>[4x]MLESKLKAPVFTATTQGDHYGEFVLEPLERGFGVTLGNPLRRILLSSIPGTAVTSVYIEDVLHEFSTIPGVKEDVVEIILNLKELVVRFLDPKMASTTLILRAEGPKEVRAGDFTPSADVEIMNPDLHIATLEEGGKLYMEVRVDRGVGYVPAERHGIKDRINAIPVDAIFSPVRRVAFQVEDTRLGQRTDLDKLTLRIWTDGSVTPLEALNQAVAILKEHLNYFANPEASLLPTPEVSKGEKRESAEEDLDLPLEELGLSTRVLHSLKEEGIESVRALLALNLKDLRNIPGIGERSLEEIRQALAKKGFTLKE;>[2x]MEIKRFGRIREVIPLPPLTEIQVESYKKALQADVPPEKRENVGIQAAFKETFPIEEGDKGKGGLVLDFLEYRIGDPPFSQDECREKDLTYQAPLYARLQLIHKDTGLIKEDEVFLGHLPLMTEDGSFIINGADRVIVSQIHRSPGVYFTPDPARPGRYIASIIPLPKRGPWIDLEVEASGVVTMKVNKRKFPLVLLLRVLGYDQETLVRELSAYGDLVQGLLDEAVLAMRPEEAMVRLFTLLRPGDPPKKDKALAYLFGLLADPKRYDLGEAGRYKAEEKLGVGLSGRTLVRFEDGEFKDEVFLPTLRYLFALTAGVPGHEVDDIDHLGNRRIRTVGELMADQFRVGLARLARGVRERMVMGSPDTLTPAKLVNSRPLEAALREFFSRSQLSQFKDETNPLSSLRHKRRISALGPGGLTRERAGFDVRDVHRTHYGRICPVETPEGANIGLITSLAAYARVDALGFIRTPYRRVKNGVVTEEVVYMTASEEDRYTIAQANTPLEGDRIATDRVVARRRGEPVIVAPEEVEFMDVSPKQVFSLNTNLIPFLEHDDANRALMGSNMQTQAVPLIRAQAPVVMTGLEERVVRDSLAALYAEEDGEVVKVDGTRIAVRYEDGRLVEHPLRRYARSNQGTAFDQRPRVRVGQRVKKGDLLADGPASEEGFLALGQNVLVAIMPFDGYNFEDAIVISEELLKRDFYTSIHIERYEIEARDTKLGPERITRDIPHLSEAALRDLDEEGIVRIGAEVKPGDILVGRTSFKGEQEPSPEERLLRSIFGEKARDVKDTSLRVPPGEGGIVVGRLRLRRGDPGVELKPGVREVVRVFVAQKRKLQVGDKLANRHGNKGVVAKILPVEDMPHLPDGTPVDVILNPLGVPSRMNLGQILETHLGLAGYFLGQRYISPVFDGATEPEIKELLAEAFNLYFGKRQGEGFGVDKREKEVLARAEKLGLVSPGKSPEEQLKELFDLGKVVLYDGRTGEPFEGPIVVGQMFIMKLYHMVEDKMHARSTGPYSLITQQPLGGKAQFGGQRFGEMEVWALEAYGAAHTLQEMLTIKSDDIEGRNAAYQAIIKGEDVPEPSVPESFRVLVKELQALALDVQTLDEKDNPVDIFEGLASKR;>MKKEVRKVRIALASPEKIRSWSYGEVEKPETINYRTLKPERDGLFDERIFGPIKDYECACGKYKRQRFEGKVCERCGVEVTRSIVRRYRMGHIELATPAAHIWFVKDVPSKIGTLLDLSATELEQVLYFNKYIVLDPKGAVLDGVPVEKRQLLTDEEYRELRYGKQETYPLPAGVDALVKDGEEVVKGQELAPGVVSRMDGVALYRFPRRVRVDYLRKERAALRIPLSAWVEKEAYRPGEVLAELSEPYLFRAEESGVVELKDLAEGHLIYLRQEEEVVARYFLPAGMTPLVVEGEIVEVGQPLAEGKGLLRLPRHMTAKEVEAEEEGDSVHLTLFLEWTEPKDYKVAPHMNVIVPEGAKVQAGEKIVAAIDPEEEVIAEAEGVVHLHEPASILVVKARVYPFEDDVEVTTGDRVAPGDVLADGGKVKSEIYGRVEVDLVRNVVRVVESYDIDARMGAEAIQELLKELDLEKLERELLEEMKHPSRARRAKARKRLEVVRAFLDSGNRPEWMILEAVPVLPPDLRPMVQVDGGRFATSDLNDLYRRLINRNNRLKKLLAQGAPEIIIRNEKRMLQEAVDAVIDNGRRGSPVTNPGSERPLRSLTDILSGKQGRFRQNLLGKRVDYSGRSVIVVGPQLKLHQCGLPKRMALELFKPFLLKKMEEKAFAPNVKAARRMLERQRDIKDEVWDALEEVIHGKVVLLNRAPTLHRLGIQAFQPVLVEGQSIQLHPLVCEAFNADFDGDQMAVHVPLSSFAQAEARIQMLSAHNLLSPASGEPLAKPSRDIILGLYYITQVRKEKKGAGMAFATPEEALAAYERGEVALNAPIVVAGRETSVGRLKFVFANPDEALLAVAHGLLDLQDVVTVRYLGRRLETSPGRILFARIVGEAVGDEKVAQELIQMDVPQEKNSLKDLVYQAFLRLGMEKTARLLDALKYYGFTLSTTSGITIGIDDAVIPEEKQRYLEEADRKLRQIEQAYEMGFLTDRERYDQVIQLWTETTEKVTQAVFKNFEENYPFNPLYVMAQSGARGNPQQIRQLCGMRGLMQKPSGETFEVPVRSSFREGLTVLEYFISSHGARKGGADTALRTADSGYLTRKLVDVAHEIVVREADCGTTNYISVPLFQMDEVTRTLRLRKRSDIESGLYGRVLAREVEALGRRLEEGRYLSLEDVHFLIKAAEAGEVREVPVRSPLTCQTRYGVCQKCYGYDLSMARPVSIGEAVGVVAAESIGEPGTQLTMRTFHTGGVAVGTDITQGLPRVIELFEARRPKAKAVISEIDGVVRIEEGEDRLSVFVESEGFSKEYKLPKDARLLVKDGDYVEAGQPLTRGAIDPHQLLEAKGPEAVERYLVDEIQKVYRAQGVKLHDKHIEIVVRQMLKYVEVTDPGDSRLLEGQVLEKWDVEALNERLIAEGKVPVAWKPLLMGVTKSALSTKSWLSAASFQNTTHVLTEAAIAGKKDELIGLKENVILGRLIPAGTGSDFVRFTQVVDQRTLKAIEEARKEAVEAKEKEAPRRPVRREQPGKGL[2x];>[2x]MAEPGIDKLFGMVDSKYRLTVVVAKRAQQLLRHRFKNTVLEPEERPKMRTLEGLYDDPNAVTWAMKELLTGRLFFGENLVPEDRLQKEMERLYPTEEEA;>[2x]TSDPVRQYLHEIGQVPLLTLEEEIDLARKVEEGMEAIKKLSEATGLDQELIREVVRAKILGTARIQKIPGLKEKPDPKTVEEVDGKLKSLPKELKRYLHIAREGEAARQHLIEANLRLVVSIAKKYTGRGLSFLDLIQEGNQGLIRAVEKFEYKRRFKFSTYATWWIRQAINRAIADQARTIRIPVHMVETINKLSRTARQLQQELGREPSYEEIAEAMGPGWDAKRVEETLKIAQEPVSLETPIGDEKDSFYGDFIPDENLPSPVEAAAQSLLSEELEKALSKLSEREAMVLKLRKGLIDGREHTLEEVGAYFGVTRERIRQIENKALRKLKYHESRTRKLRDFLE;>MKEFRPGDKVVLPPYGVGVVAGIAQRSVSGVSRAYYQVDFPGSRSKAYVPVEAPHSVGLRKALAPEEVPVILDLLKNGRMPLPKQWAARHRKTSEILADGNPYRIAQMAGQLRAWEVERGLPDLDRQALRRAIHLLAEEVAQSLEITVQEAKRLFEEAWGEELN[2x]

CarD, first identified as a regulator of ribosomal RNA (rRNA) transcription in Mycobacterium tuberculosis (Mtb), is a transcriptional activator widely distributed among bacterial species, including Thermus species, but is absent in Eco. CarD is a global regulator that is an essential protein in Mtb, the causative agent of tuberculosis. Crystal structures of Tth and Mtb CarD reveal an N-terminal domain with a Tudor-like fold (CarD-RID, RNAP interacting domain) in common with the Eco transcription repair coupling factor (TRCF)-RID, and a helical C-terminal domain (CarD-CTD). The structural results, combined with supporting biochemical studies, establish that the CarD-RID makes a protein/protein interaction with the RNAP β1-lobe, thereby positioning the CarD-CTD and a conserved Trp residue to interact with the upstream edge of the transcription bubble, using a wedge mechanism to prevent collapse of the transcription bubble.

To resolve these ambiguities, we determined crystal structures of Thermus aquaticus (Taq) transcription initiation complexes (RPo) containing CarD. Crystals of CarD transcription activation complexes were prepared by soaking Tth CarD into Taq Δ1.1σA-holoenzyme/us-fork (−12 bp) or full RPo crystals. Analysis of the diffraction data indicated high occupancy of one CarD molecule bound to each of two RNAP/promoter complexes in the asymmetric unit of the crystal lattice. The structures of CarD transcription activation complexes were refined to 4.4 and 4.3 Å-resolution, respectively. The protein/protein and protein/nucleic acid interactions were essentially identical among all of the four crystallographically independent complexes, so the more complete and higher resolution CarD/RPo structure is described here. The structures show that CarD interacts with the unique DNA topology of the upstream double-stranded/single-stranded (ds/ss) DNA junction of the transcription bubble. CarD interacts exclusively at the upstream junction of the transcription bubble.>[2x]MSDIITTAFEVRPLTSALGAEIHGVRLEDITDADFAELRRLLLKHLVIFIPDQEGWSAESRIAFGRRFGELEEHAYLPHLDGHPQIQIIDSEQNGKIPIWHTDMTYAPNPPIGSVLQIVDGPAQGGDTM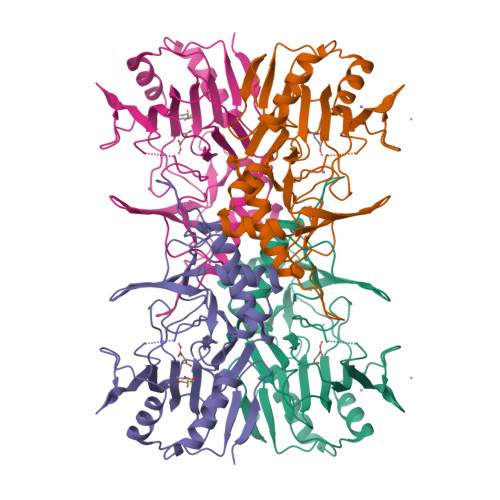WSNQYLAYEGLSAPLRDLLDGLTAVHSIHIPGLDSQAEHPVVRVHPETGRRALFVNRAHTSHIAQLNRNESDALLQYLYRFSTSPEFTCRYQWRPGSVAIWDNRVTQHYAVDDYSEHRRGLRVVVLGDTPSGDKPRWDHYRPVPGQRYVPDWVNAKEAYGKLENLYFQ> PENLVVYNDGADQRAAEYLADRLAC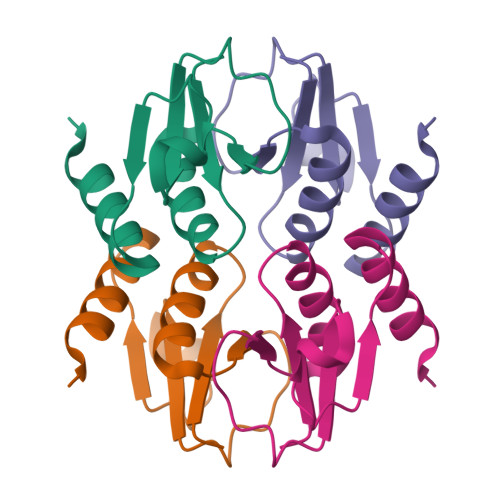PTINNARKFDYSNVKNVYAVGGNKEQYTSYLTTLIAGSTRYTTMQAVLDYIKNLK>[2x]EVDPRLYFENRSKFIQDQKDKGINPYPHKFERTISIPEFIEKYKDLGNGEHLEDTILNITGRIMRVSASGQKLRFFDLVGDGEKIQVLANYSFHNHEKGNFAECYDKIRRGDIVGIVGFPGKSKKGELSIFPKETILLSACLHMLPMKYGLKDTEIRYRQRYLDLLINESSRHTFVTRTKIINFLRNFLNERGFFEVETPMMNLIAGGANARPFITHHNDLDLDLYLRIATELPLKMLIVGGIDKVYEIGKVFRNEGIDNTHNPEFTSCEFYWAYADYNDLIKWSEDFFSQLVYHLFGTYKISYNKDGPENQPIEIDFTPPYPKVSIVEEIEKVTNTILEQPFDSNETIEKMINIIKEHKIELPNPPTAAKLLDQL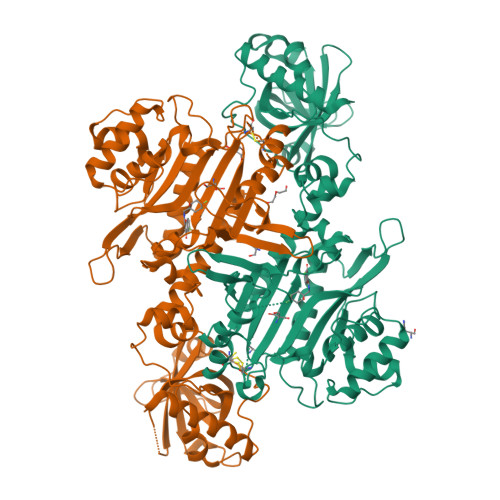ASHFIENKYNDKPFFIVEHPQIMSPLAKYHRTKPGLTERLEMFICGKEVLNAYTELNDPFKQKECFKLQQKDREKGDTEAAQLDSAFCTSLEYGLPPTGGLGLGIDRITMFLTNKNSIKDVILFPTMRPAN benzene-1,2,4-tricarboxylic acid | C9 H6 O6 | 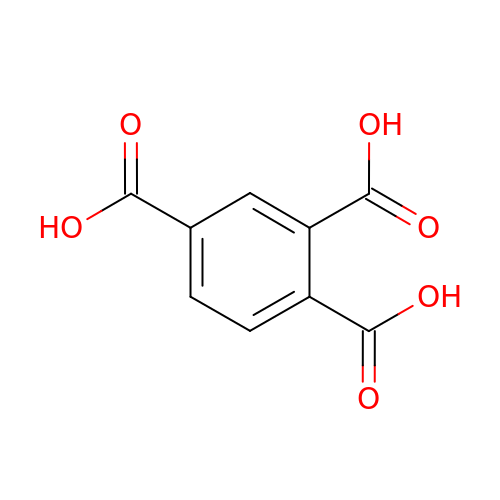ARCGXLSVLAOJQL-UHFFFAOYSA-N> IVGGTNSSWGEWPWQVSLQVKLTAQRHLCGGSLIGHQWVLTAAHCFDGLPLQDVWRIYSGILNLSDITKDTPFSQIKEIIIHQNYKVSEGNHDIALIKLQAPLNYTEFQKPISLPSKGDTSTIYTNCWVTGWGFSKEKGEIQN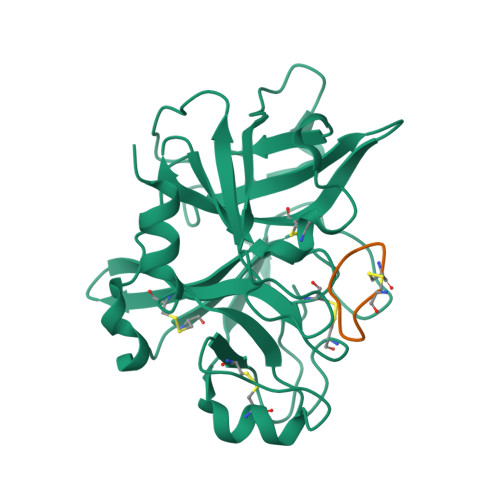ILQKVNIPLVTNEECQKRYQDYKITQRMVCAGYKEGGKDACKGDSGGPLVCKHNGMWRLVGITSWGEGCARREQPGVYTKVAEYMDWILEKTQS;> CPAYSXYLDC> MGNICVGGSRMAHQVNSPDRVSNNSGDEDNVTSSQLLSVRHQLAESAGLPRDQHEFVSSQAPQSLRNRYNNLYSH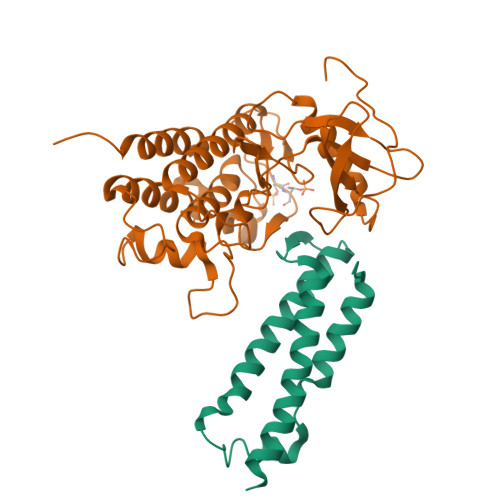TQRTLDMADMQHRYMTGASGINPGMLPHENVDDMRSAITDWSDMREALQHAMGIHADIPPSPERFVATMNPSGSIRMSTLSPSPYRNWQ;> MGSKYSKATNSINDALSSSYLVPFESYRVPLVDLEEATNNFDHKFLIGHGVFGKVYKGVLRDGAKVALKRRTPESSQGIEEFETEIETLSFCRHPHLVSLIGFCDERNEMILIYKYMENGNLKRHLYGSDLPTMSMSWEQRLEICIGAARGLHYLHTRAIIHRDVKSINILLDENFVPKITDFGISKKGTELDQTHLSTVVKGTLGYIDPEYFIKGRLTEKSDVYSFGVVLFEVLCARSAIVQSLPREMVNLAEWAVESHNNGQLEQIVDPNLADKIRPESLRKFGDTAVKCLALSSEDRPSMGDVLWKLEYALRLQESVI> MLGLGGAATRQLTFQTSSPAHLTMPYVMPGDGEVVGVGEPVAIRFDENIADRGAAEKAIKITTNPPVEGAFYWLNNREVRWRPEHFWKPGTAVDVAVNTYGVDLGEGMFGEDNVQTHFTIGDEVIATADDNTKILTVRVNGEVVKSMPTSMGKDSTPTANGIYIVGSRYKHIIMDSSTYGVPVNSPNGYRTDVDWATQISYSGVFVHSAPWSVGA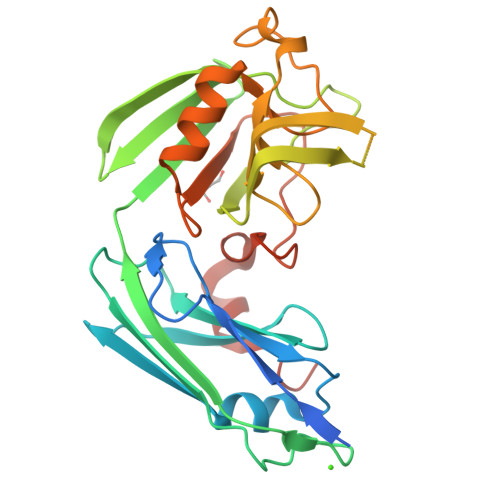QGHTNTSHGCLNVSPSNAQWFYDHVKRGDIVEVVNTVGGTLPGIDGLGDWNIPWDQWRAGNAKALEHHHHHH> GGTIARTIVLQESIGKGRFGEVWRGKWRGEEVAVKIFSSREERSWFREAEIYQTVMLRHENILGFIAADNKDNGTWTQLWLVSDYHEHGSLFDYLNRYTVTVEGMIKLALSTASGLAHLHMEIVGTQGKPAIAHRDLKSKNILVKKNGTCCIADLGLAVRHDSATDTIDIAPNHRVGTKRYMAPEVLDDSINMKHFESFKRADIYAMGLVFWEIARRCSIGGIHEDYQLPYYDLVPSDPSVEEMRKVVCEQKLRPNIPNRWQSCEALRVMAKIMRECWYANGAARLTALRIKKTLSQLSQQEG

TGF-β is a key regulator in various types of cancer, exerting its effects through the intracellular domain (ICD) of TGF-β receptor I (TβRI; Boguslawska et al., 2019). Activation of TGF-β signalling involves specific type I and type II serine/threonine kinase receptors, ultimately leading to the phosphorylation of Smad proteins, notably Smad2 and Smad3, to orchestrate gene expression. The crystal structure of the intracellular domain of transforming growth factor β type I receptor (TβR1) in complex with the competitive inhibitor SB505124 is presented.

The TβRI–SB505124 complex closely resembles the TβRI kinase conformation observed in the TβRI–SB431542 complex. Molecular-docking studies and comparative modelling have also shown that SB505124 aligns more favourably within the ALK5 binding site compared with other ALK receptors, forming more stable interactions and supporting its structural selectivity. Clear electron density was observed for SB505124, with a heterocyclic ring structure (pyridine, pyrimidine and benzene rings) similar to SB431542 (pyridine and benzodioxole rings); both of them act as a type I kinase inhibitor by occupying the ATP-binding region and adjacent hydrophobic sites near the hinge region, which is the linker between the N- and C-terminal kinase lobes. The position of the pyridinyl ring adjacent to the gatekeeper residue is further stabilized by hydrophobic interactions with Leu260 and Leu278. Two hydrogen bonds link SB505124 with ICD: one is between the benzodioxole O atom of SB505124 and the amide N atom of His283 from the hinge region, a feature that is common to many ATP-competitive kinase inhibitors, while the second hydrogen bond is between Leu332 and the imidazole ring of SB505124, which is also stabilized by Val219 through hydrophobic interactions.4-methyl-7-(2-{3-[(methylamino)methyl]phenyl}ethyl)quinolin-2-amine | C20 H23 N3 | 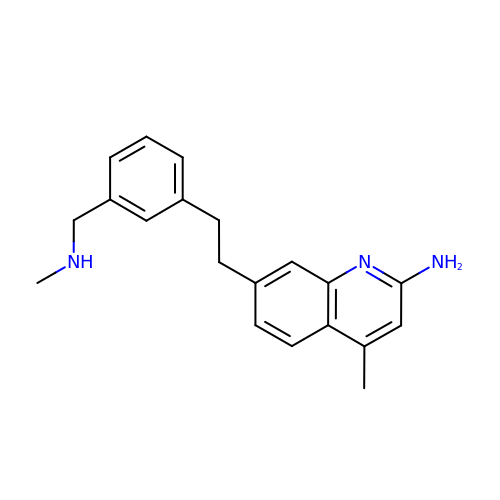VJMAXFIJCSRVHO-UHFFFAOYSA-N> SNATFLELVEVPCNSVHVQGVMTPNQMVKVTGAGWDNGVLEFYVTRPTKTGGDTSRSHLASIMCYSKDIDGVPSDKAGKCFLKRFSGEDSSEID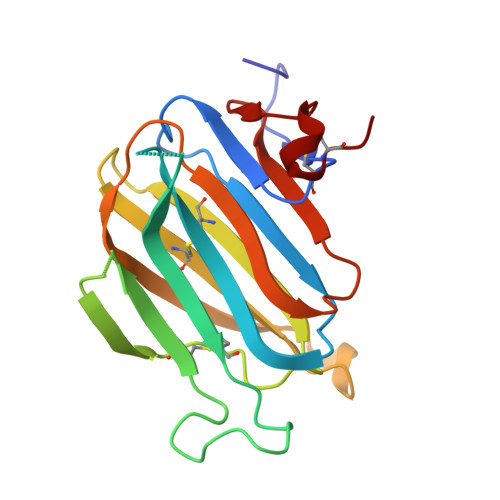EKEVSLPIKSHNDAFMFVCSSNDGSALQCDVFALDNTNSNDGWKVNTVDLGVSVSPDLAFGLTADGVKVKKLYASSGLTAINDDPSLGCKA>KFDDVCGCDEARAELEEIVDFLKDPTKYESLGGKLPKGVLLTGPPGTGKTLLARATAGEAGVDFFFMSGSEFDEVYVGVGAKRIRDLFAQARSRAPAIIFIDQLDAIGGKRNPKDQAYAKQTLNQLLVELDGFSQTSGIIIIGATNFPEALDKALTRPGRFDKVVNVDLPDVRGRADILKHHMKKITLADNVDPTIIARGTPGLSGAELANLVNQAAVYACQKNAVSVDMSHFEWAKDKILMGAERKTMVLTDAARKATAFHEAGHAIMAKYTNGATPLYKATILPRGRALGITFQLPEMDKVDITKRECQARLDVCMGGKIAEELIYGKDNTTSGCGSDLQSATGTARAMVTQYGMSDDVGPVNLSEEWESWSNKIRDIADNEVIELLKDSEERARRLLTKKNVELHRLAQGLIEYETLDAHEIEQ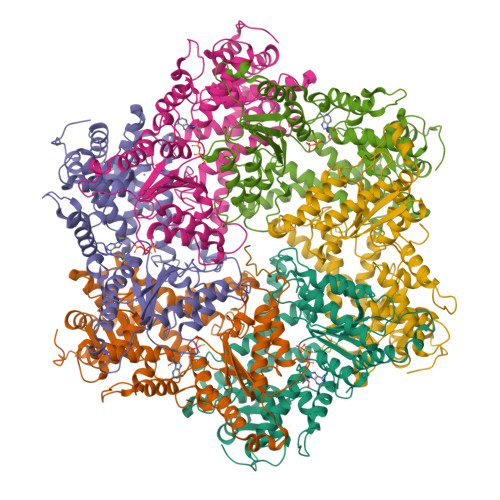VCKGEKLAKLKT[6x]>MHRYSRTGKHRWTVRALAVLFTALLGLTQWTAPASAHGSVINPATRNYGCWLRWGHDHLNPNMQYEDPMCWQAWQDNPNAMWNWNGLYRDWVGGNHRAALPDGQLCSGGLTEGGRYRSMDAVGPWKTTDVNNTFTIHLYDQASHGADYFLVYVTKQGFDPTTQPLTWD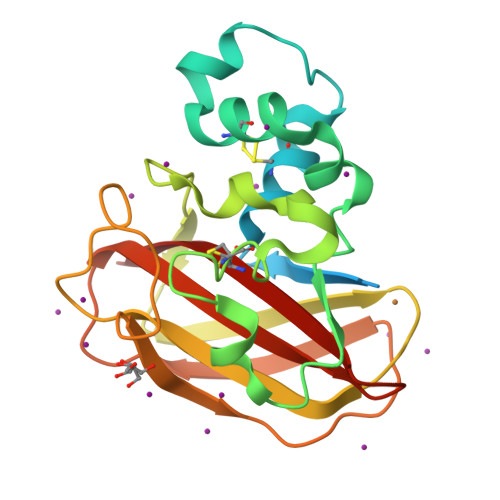SLELVHQTGSYPPAQNIQFTVHAPNRSGRHVVFTIWKASHMDQTYYLCSDVNFV[2x]(2S,5R)-1-formyl-N'-[(3R)-pyrrolidine-3-carbonyl]-5-[(sulfooxy)amino]piperidine-2-carbohydrazide 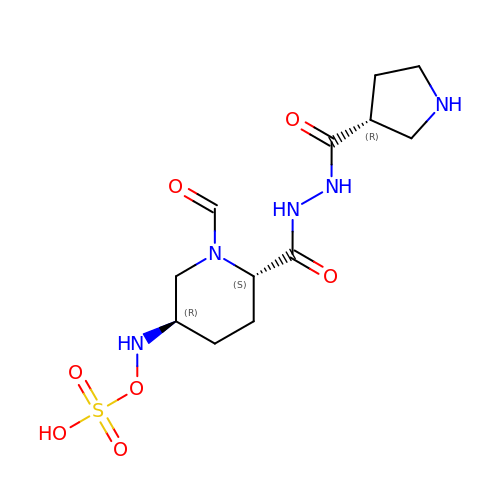| C12 H21 N5 O7 S | MPNPDELHXLJIKQ-BBBLOLIVSA-N> MKLRAEDVLANGTSRHKVQIDMERQVQIAKDLLAQKKFLEAAKRCQQTLDSLPKDGLLPDPELFTIFAQAVYNMEVQNSGNLFGDALLAGDDGS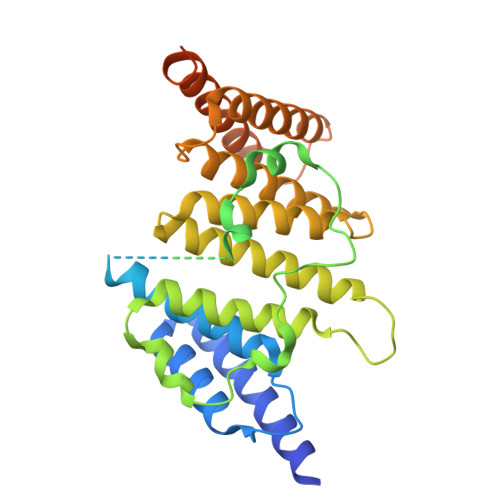GSESESEPESDVSNGEEGNENGQTEIPNSRMFQFDQEEEDLTGDVDSGDSEDSGEGSEEEEENVEKEEERLALHELANFSPANEHDDEIEDVSQLRKSGFHIYFENDLYENALDLLAQALMLLGRPTADGQSLTENSRLRIGDVYILMGDIEREAEMFSRAIHHYLKALGYYKTLKPAEQVTEKVIQAEFLVCDALRWVDQVPAKDKLKRFKHAKALLEKHMTTRPKDSELQQARLAQIQDDIDEVQENQQHGSKRPLSQPTTSIGFPALEKPLGDFNDLSQLVKKKPRRHLEHHHHHH(1R,2S,3R)-5-[(E)-2-[(1R,3aS,7aR)-7a-methyl-1-[(2R)-6-methyl-6-oxidanyl-heptan-2-yl]-1,2,3,3a,6,7-hexahydroinden-4-yl]ethenyl]-2-(3-oxidanylpropyl)cyclohex-4-ene-1,3-diol 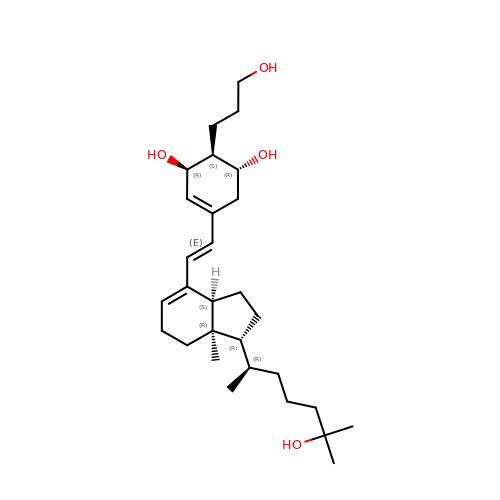| C29 H48 O4 | FSKKMLBYNCANGG-IATMLIOWSA-N>[2x]MSEWWKEAVVYQIYPRSFYDANGDGFGDLQGVIQKLDYIKNLGADVIWLSPVFDSPQDDNGYDISDYKNMYEKFGTNEDMFQLIDEVHKRGMKIVMDLVVNHTSDEHAWFAESRKSKDNPYRDYYLWKDPKPDGSEPNNWGSIFSGSAWTYDEGTGQYYLHYFSKKQPDLNWENEAVRREVYDVMRFWMDRGVDGWRMDVIGSISKYTDFPDYETDHSRSYIVGRYHSNGPRLHEFIQEMNREVLSHYDCMTVGEANGSDIEEAKKYTDASRQELNMIFTFEHMDIDKEQNSPNGKWQIKPFDLIALKKTMTRWQTGLMNVGWNTLYFENHDQPRVISRWGNDRKLRKECAKAFATVLHGMKGTPFIYQGEEIGMVNSDMPLEMYDDLEIKNAYRELVVENKTMSEKEFVKAVMIKGRDHARTPMQWDAGKHAGFTAGDPWIPVNSRYQDINVK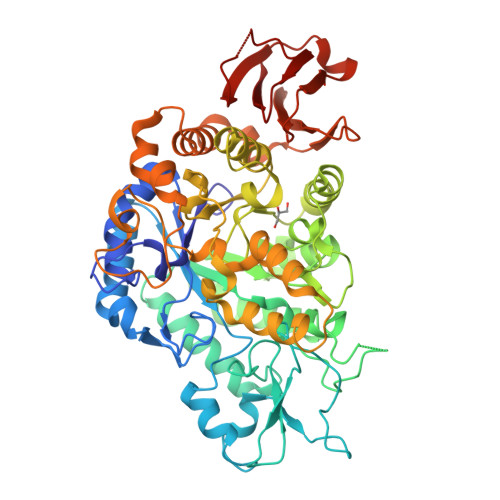ESLEDQDSIFFYYQKLIQLRKQYKIMIYGDYQLLQENDPQVFSYLREYRGEKLLVVVNLSEEKALFEAPPELIHERWKVLISNYPQERADLKSISLKPYEAVMGISI> MNADEWMTTFRENIAQTWQQPEHYDLYIPAITWHARFAYDKEKTDRYNERPWGGGFGLSRWDEKGNWHGLYAMAFKDSWNKWE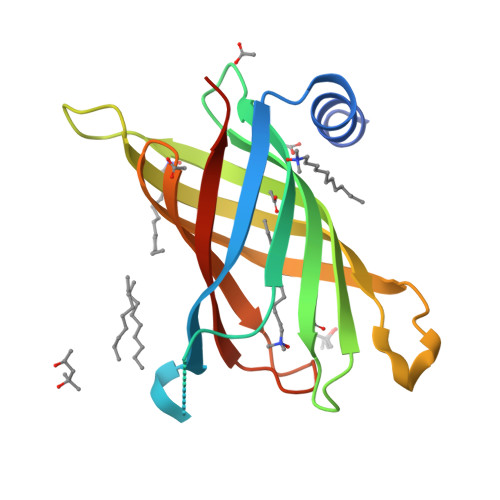PIAGYGWESTWRPLADENFHLGLGFTAGVTARDNWNYIPLPVLLPLASVGYGPVTFQMTYIPGTYNNGNVYFAWMRFQFLEHHHHHH> MQNGYTYEDYQDTAKWLLSHTEQRPQVAVI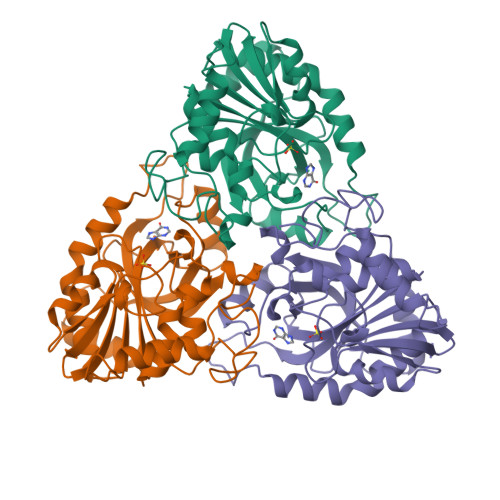CGSGLGGLVNKLTQAQTFDYSEIPNFPESTVPGHAGRLVFGILNGRACVMMQGRFHMYEGYPFWKVTFPVRVFRLLGVETLVVTNAAGGLNPNFEVGDIMLIRDHINLPGFSGENPLRGPNEERFGVRFPAMSDAYDRDMRQKAHSTWKQMGEQRELQEGTYVMLGGPNFETVAECRLLRNLGADAVGMSTVPEVIVARHCGLRVFGFSLITNKVIMDTESQGKANHEEVLEAGKQAAQKLEQFVSLLMASI> GSMPMYEVQWKVVEESNGNNYSYIDPTQLPYDHKWEFPRNRLSFGKTLGAGAFGKVVEATAQGLIKSDAAMTVAVKMLKPSAHSTEREALMSELKVLSYLGNHENIVNLLGACTHGGPTLVITEYCCYGDLL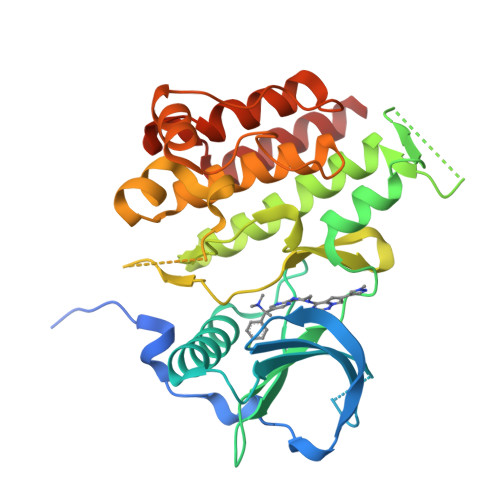NFLRRKRDEFVPYKVAPEDLYKDFLTLEHLLSFSYQVAKGMAFLASKNCIHRDLAARNILLTHGNITKICDFGLARDIKNDSNYVDKGNARLPVKWMAPESIFNSVYTFESDVWSYGIFLWELFSLGSSPYPGMPVDSKFYKMIKEGFRMSSPEYAPAEMYDIMKTCWDADPDKRPTFKQIVQDIEKQISESTNH>[3x]DYKFWYTQPVPKINDEFNESVNEPFISDNKVEDVRKDEYKLPPGYSWYVCDVKDEKDRSEIYTLLTDNYVEDDDNIFRFNYSAEFLLWALTSPNY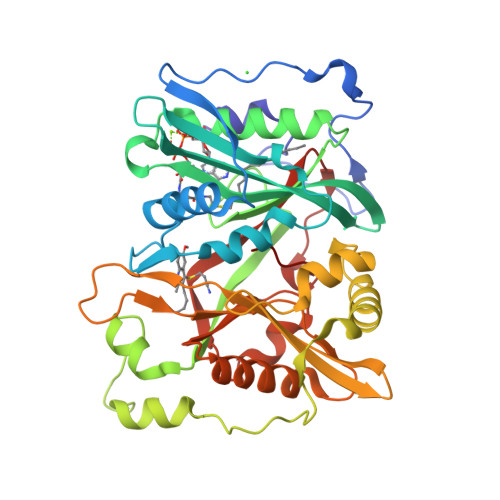LKTWHIGVKYDASNKLIGFISAIPTDICIHKRTIKMAEVNFLCVHKTLRSKRLAPVLIKEITRRINLENIWQAIYTAGVYLPKPVSDARYYHRSINVKKLIEIGFSSLNSRLTMSRAIKLYRVEDTLNIKNMRLMKKKDVEGVHKLLGSYLEQFNLYAVFTKEEIAHWFLPIENVIYTYVNEENGKIKDMISFYSLPSQILGNDKYSTLNAAYSFYNVTTTATFKQLMQDAILLAKRNNFDVFNALEVMQNKSVFEDLKFGEGDGSLKYYLYNWKCASFAPAHVGIVLL>[2x]MASGSASSAQTPGLMSWLPPSNQLSPEARSVLDRMDAAKAPEFNGDLVRQRAFYQQFNDDRLVEMRRVFRTRERHETLNAVHVQVVEPADGVSARNRDRVLINVHGGAFMWGAGSGALVEAIPIAATMGVSVVTVDYRLAPENRYPAASEDVTAVYRALLERYPAANIGIFGCSAGGVITAQAVTWIRREGLPRPGAIGTLCGTGAPYSGDSPYLAGVVPVGPGVKAPPLPGLLPTAYMEGVGADDARAYPLTSDAETVFMPPTLLLAGGRDFAVSALSLAHRRLARAGVDSELHLFDGLPHAFFVWPDMPESLEAYALIAGFFDSRLGLTPSSSIPTPRSPSHHHHHH

Among them, a new esterase PMGL2 belonging to the hormone sensitive lipase (HSL, EC 3.1.1.79) family (family IV lipases) was produced and biochemically characterized. The unique feature of this enzyme is the presence of a cysteine residue in the GCSAG motif which surrounds the conserved catalytic serine. Three-dimensional structures of subunits of wtPMGL2 and its mutant variant mPMGL2 were found to be quite similar (see Methods section). Both of them had a typical α/β bacterial HSL-like fold, consisting of two canonical domains ‒ a CAP-domain and a catalytic domain. The active site of PMGL2 consists of a catalytic triad of conserved His302, Asp272 and Ser174.

In order to reveal the structural features associated with this new sequence motif, we have crystallized the wild type PMGL2 (wtPMGL2) and determined its 3D structure. It was the third structure of an enzyme from the GTSAG motif subfamily established and the first one with the GCSAG variant. Two cysteine residues, Cys173 and Cys202, were found in the active site of wtPMGL2, where Cys173 was a part of the 172GCSAG176 motif possessing the catalytic serine residue. The side chains of both cysteines were clearly visible in an electron density with a distance between their Cβ atoms of 5.2 Å. However, these residues were not disulfide bonded in wtPMGL2 structure as followed from the electron density. Moreover, structural studies and MALDI analysis did not reveal the presence of the disulfide bond between Cys202 and Cys173, however, it can be speculated that their proximity may allow for disulfide bonding in appropriate conditions and upon small movement of the main chain in the active site region. In wtPMGL2, Tyr208 residue has two conformations of its side chain with relatively poor density. The region 216–237 also possesses the same conformation in both structures with, however, an absence of electron density for the residues 221–226 of one subunit of wtPMGL2 coupled with a high temperature factor and the poor electron density in this region in both structures. Interestingly, PEG molecule was found in the active site of mPMGL2 (but not in wtPMGL2).AMINOGUANIDINE | C H6 N4 | 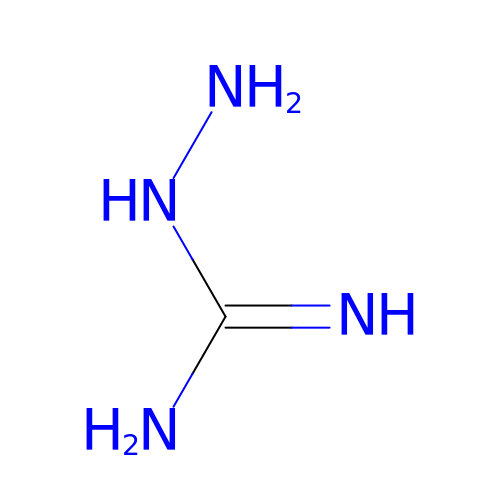HAMNKKUPIHEESI-UHFFFAOYSA-N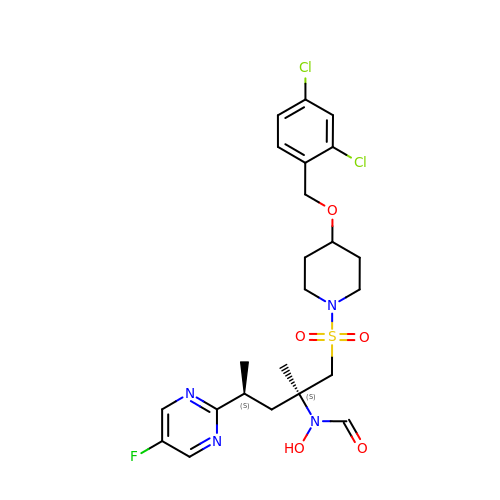N-[(2S,4S)-1-({4-[(2,4-dichlorobenzyl)oxy]piperidin-1-yl}sulfonyl)-4-(5-fluoropyrimidin-2-yl)-2-methylpentan-2-yl]-N-hydroxyformamide | C23 H29 Cl2 F N4 O5 S | YSYXAGMNRKARQB-HJPURHCSSA-N~{N}-[3-(4-fluorophenyl)prop-2-ynyl]-2-(trifluoromethyl)pyridin-4-amine 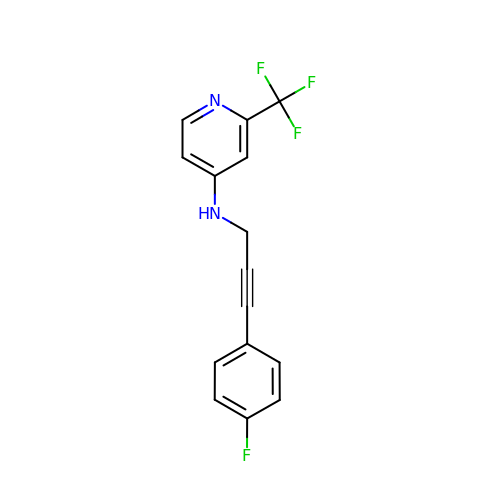| C15 H10 F4 N2 | LOCKKGFITVJYKW-UHFFFAOYSA-N>[2x]MTGPILSGLDPRFERTLYAHVGKEGSWTLDYYLRHGGYETAKRVLKEKTPDEVIEEVKRSGLRGRGGAGFPTGLKWSFMPKDDGKQHYLICNADESEPGSFKDRYILEDVPHLLIEGMILAGYAIRATVGYIYVRGEYRRAADRLEQAIKEARARGYLGKNLFGTDFSFDLHVHRGAGAYICGEETALMNSLEGLRANPRLKPPFPAQSGLWGKPTTINNVETLASVVPIMERGADWFAQMGTEQSKGMKLYQISGPVKRPGVYELPMGTTFRELIYEWAGGPLEPIQAIIPGGSSTPPLPFTEEVLDTPMSYEHLQAKGSMLGTGGVILIPERVSMVDAMWNLTRFYAHESCGKCTPCREGVAGFMVNLFAKIGTGQGEEKDVENLEALLPLIEGRSFCPLADAAVWPVKGSLRHFKDQYLALAREKRPVPRPSLWR;>MGFFDDKQDFLEETFAKYPPEGRRAAIMPLLRRVQQEEGWIRPERIEEIARLVGTTPTEVMGVASFYSYYQFVPTGKYHLQVCATLSCKLAGAEELWDYLTETLGIGPGEVTPDGLFSVQKVECLGSCHTAPVIQVNDEPYVECVTRARLEALLAGLRAGKRLEEIELPGKCGHHVHEVEV[2x];>[2x]MVRVKVNDRIVEVPPGTSVMDAVFHAGYDVPLFCSEKHLSPIGACRMCLVRIGLPKKGPDGKPLLNEKGEPEIQWQPKLAASCVTAVADGMVVDTLSDVVREAQAGMVEFTLLNHPLDCPTCDKGGACELQDRTVEYGLYEKYYQKGPLELPVYTRFEFTRRHVDKHHPLSPFVILDRERCIHCKRCVRYFEEVPGDEVLDFIERGVHTFIGTMDFGLPSGFSGNITDICPVGALLDLTARFRARNWEMEETPTTCALCPVGCGITADTRSGELLRIRAREVPEVNEIWICDAGRFGHEWADQNRLKTPLVRKEGRLVEATWEEAFLALKEGLKEARGEEVGLYLAHDATLEEGLLASELAKALKTPHLDFQGRTAAPASLFPPASLEDLLQADFALVLGDPTEEAPILHLRLSEFVRDLKPPHRYNHGTPFADLQIKERMPRRTDKMALFAPYRAPLMKWAAIHEVHRPGEEREILLALLGDKEGSEMVAKAKEAWEKAKNPVLILGAGVLQDTVAAERARLLAERKGAKVLAMTPAANARGLEAMGVLPGAKGASWDEPGALYAYYGFVPPEEALKGKRFVVMHLSHLHPLAERYAHVVLPAPTFYEKRGHLVNLEGRVLPLSPAPIENGEAEGALQVLALLAEALGVRPPFRLHLEAQKALKARKVPEAMGRLSFRLKELRPKERKGAFYLRPTMWKAHQAVGKAQEAARAELWAHPETARAEALPEGAQVAVETPFGRVEARVVHREDVPKGHLYLSALGPAAGLRVEGRVLVPAGGEA;>MREEFLEEIPLDAPPEEAKELRTEVMTLNVGPQHPSTHGVLRLMVTLSGEEVLEVVPHIGYLHTGFEKTMEHRTYLQNITYTPRMDYLHSFAHDLAYALAVEKLLGAVVPPRAETIRVILNELSRLASHLVFLGTGLLDLGALTPFFYAFRERETILDLFEWVTGQRFHHNYIRIGGVKEDLPEEFVPELKKLLEVLPHRIDEYEALFAESPIFYERARGVGVIPPEVAIDLGLTGGSLRASGVNYDVRKAYPYSGYETYTFDVPLGERGDVFDRMLVRIREMRESVKIIKQALERLEPGPVRDPNPQITPPPRHLLETSMEAVIYHFKHYTEGFHPPKGEVYVPTESARGELGYYIVSDGGSMPYRVKVRAPSFVNLQSLPYACKGEQVPDMVAIIASLDPVMGDVDR[2x];>MRLERVLEEARAKGYPIEDNGLGNLWVVLPRERFKEEMAHYKAMGFNFLADIVGLDYLTYPDPRPERFAVVYELVSLPGWKDGDGSRFFVRVYVPEEDPRLPTVTDLWGSANFLEREVYDLFGIVFEGHPDLRKILTPEDLEGHPLRKDYPLGETPTLFREGRYIIPAEFRAALTGKDPGLTFYKGGSRKGYRSLWADLKKAREVKG[2x];>MALKDLFERDVQELEREGILFTTLEKLVAWGRSNSLWPATFGLACCAIEMMASTDARNDLARFGSEVFRASPRQADVMIVAGRLSKKMAPVMRRVWEQMPDPKWVISMGACASSGGMFNNYAIVQNVDSVVPVDVYVPGCPPRPEALIYAVMQLQKKVRGQAYNERGERLPPVAAWKRTRG[2x];>MSASSERELYEAWVELLSWMREYAQAKGVRFEKEADFPDFIYRMERPYDLPTTIMTASLSDGLGEPFLLADVSPRHAKLKRIGLRLPRAHIHLHAHYEPGKGLVTGKIPLTKERFFALADRAREALAFA[2x];>[2x]MTLKALAQSLGITLKYLFSKPVTVPYPDAPVALKPRFHGRHVLTRHPNGLEKCIGCSLCAAACPAYAIYVEPAENDPENPVSAGERYAKVYEINMLRCIFCGLCEEACPTGAIVLGYDFEMADYEYSDLVYGKEDMLVDVVGTKPQRREAKRTGKPVKVGYVVPYVRPELEGFKAPTEGGKR;>MAPIQEYVGTLIYVGVALFIGVAALLVGALLGPKKPGRAKLMPYESGNDPAGEVKRFPVHFYVVAMLFILFDVEVAFLWPYAVSAGGLGLYGFLGVLAFTLLLFVGFLYEWWKGVMRWH[2x];>[2x]MTWSYPVDPYWMVALKALLVVVGLLTAFAFMTLIERRLLARFQVRMGPNRVGPFGLLQPLADAIKSIFKEDIVVAQADRFLFVLAPLISVVFALLAFGLIPFGPPGSFFGYQPWVINLDLGILYLFAVSELAVYGIFLSGWASGSKYSLLGSLRSSASLISYELGLGLALLAPVLLVGSLNLNDIVNWQKEHGWLFLYAFPAFLVYLIASMAEAARTPFDLPEAEQELVGGYHTEYSSIKWALFQMAEYIHFITASALIPTLFLGGWTMPVLEVPYLWMFLKIAFFLFFFIWIRATWFRLRYDQLLRFGWGFLFPLALLWFLVTALVVALDLPRTYLLYLSALSFLVLLGAVLYTPKPARKGGGA;>[2x]MSLLEGLALFLLLLSGVLVVTLRNAIHAALALILNFLVLAGVYVALDARFLGFIQVIVYAGAIVVLFLFVIMLLFAAQGEIGFDPLVRSRPLAALLALGVAGILAAGLWGLDLAFTQDLKGGLPQALGPLLYGDWLFVLLAVGFLLMAATVVAVALVEPGKASRAKEAEKREEVAR;>[2x]MSYLLTSALLFALGVYGVLTRRTAILVFLSIELMLNAANLSLVGFARAYGLDGQVAALMVIAVAAAEVAVGLGLIVAIFRHRESTAVDDLSELRG;>[2x]MALLGTILLPLLGFALLGLFGKRMREPLPGVLASGLVLASFLLGAGLLLSGGARFQAEWLPGIPFSLLLDNLSGFMLLIVTGVGFLIHVYAIGYMGGDPGYSRFFAYFNLFIAMMLTLVLADSYPVMFIGWEGVGLASFLLIGFWYKNPQYADSARKAFIVNRIGDLGFMLGMAILWALYGTLSISELKEAMEGPLKNPDLLALAGLLLFLGAVGKSAQIPLMVWLPDAMAGPTPVSALIHAATMVTAGVYLIARSSFLYSVLPDVSYAIAVVGLLTAAYGALSAFGQTDIKKIVAYSTISQLGYMFLAAGVGAYWVALFHVFTHAFFKALLFLASGSVIHALGGEQDVRKMGGLWKHLPQTRWHALIGALALGGLPLLSGFWSKDAILAATLTYPFGGVGFYVGALLVAVLTAMYAMRWFVLVFLGEERGHHHPHEAPPVMLWPNHLLALGSVLAGYLALPHPLPNVLEPFLKPALAEVEAHHLSLGAEWGLIALSAAVALLGLWAGFVFFQRKVFPAWYLAFEAASREAFYVDRAYNALIVNPLKALAEALFYGDRGLLSGYFGLGGAARSLGQGLARLQTGYLRVYALLFVLGALLLLGVMRW;>MVVLAVLLPVVFGALLLLGLPRALGVLGAGLSFLLNLYLFLTHPGGVAHAFQAPLLPGAGVYWAFGLDGLSALFFLTIALTVFLGALVARVEGRFLGLALLMEGLLLGLFAARDLLVFYVFFEAALIPALLMLYLYGGEGRTRALYTFVLFTLVGSLPMLAAVLGARLLSGSPTFLLEDLLAHPLQEEAAFWVFLGFALAFAIKTPLFPLHAWLPPFHQENHPSGLADALGTLYKVGVFAFFRFAIPLAPEGFAQAQGLLLFLAALSALYGAWVAFAAKDFKTLLAYAGLSHMGVAALGVFSGTPEGAMGGLYLLAASGVYTGGLFLLAGRLYERTGTLEIGRYRGLAQSAPGLAALALILFLAMVGLPGLSGFPGEFLTLLGAYKASPWLAALAFLSVIASAAYALTAFQKTFWEEGGSGVKDLAGAEWGFALLSVLALLLMGVFPGYFARGLHPLAEAFAKLLGGGA[2x];>MTLAILAVFSVALTLLGFVLPPQGVKRATLLGLALALASLLLTWGKPFAFGPYAVDGVSQVFTLLALLGALWTVGLVRSGRFEFYLLVLYAALGMHLLASTRHLLLMLVALEALSLPLYALATWRRGQGLEAALKYFLLGALAAAFFLYGAALFYGATGSLVLGAPGEGPLYALALGLLLVGLGFKAALAPFHFWTPDVYQGSPTPVVLFMATSVKAAAFAALLRVAAPPEALALLVALSVVVGNLAALAQKEAKRLLAYSSIAHAGYMALALYTGNAQALGFYLLTYVLATGLAFAVLSQISPDRVPLEALRGLYRKDPLLGLAFLVAMLSLLGLPPLAGFWGKYLAFAEAARAGAWGVLVLALVTSAVSAYYYLGLGLAVFARPEETPFRPGPPWARAAVVAAGVLLLALGLLPGLVLPALAAGG[2x];>MVRVGMRAAPRVSLEALKAALGGLKLSEAKVYLITDWQDKRDQARYALLLHTGKKDLLVPDAFGPAFPGGEEALSELVGLLLAQGARRFYEAVVSPGEMTALLDLPPEELLKRVMAIANPTDPGIYLKRAA[2x]

Complex I (NADH:ubiquinone (UQ) oxidoreductase) is the first and the largest enzyme of the respiratory chain, catalysing the transfer of two electrons from NADH to UQ, coupled to the translocation of four protons across the bacterial or inner mitochondrial membrane. In bacterial complex I the 14 “core” subunits, necessary and sufficient for complex I function, are shared equally between the peripheral and membrane arms, together forming an L-shaped molecule. All known co-factors of complex I reside in the PA: the primary electron acceptor flavin-mononucleotide (FMN) is connected by the redox chain of seven Fe–S clusters to the quinone-binding site (Q-site) at the interface with the membrane domain. In this work we address this question by building and analyzing atomic structures of nine different conformational states of complex I, which were obtained by X-ray crystallography and single-particle cryo-EM.

Aureothin, pyridaben and piericidin A are the most potent inhibitors of T. thermophilus complex I, while rotenone is less effective than it is with mammalian enzyme. All Q-like ligands studied here display a similar pattern of interactions at the deepest end of the Q-cavity, with the headgroup about 12 Å away from cluster N2. A shared feature between all ligands bound in the Q-site is a hydrogen bond interaction of a ketone group from the quinone ring with the conserved and essential for complex I activity Y87416,36. Finally, pyridaben seems to be stabilized only through the conserved interaction with Y874, although its proximity to Q334 (3–4 Å) could facilitate an interaction with both the thioether and chloride groups. In addition, the tert-butyl group points towards a small hydrophobic cavity and the 4-tert-butylcyclohexyl moiety is surrounded by non-polar residues, completing its accommodation. In these structures quinone-like compounds are bound in the main “deep” site within the cavity, where quinone can effectively accept electrons from cluster N2. Most dramatic changes are caused by DQ binding, whilst Q-like inhibitors alter complex I conformation consistently in a similar way but to a lesser degree, to states intermediate between CXIINT and CXIDQ. The overlap analysis (OA) (technique described below) shows that transitions from CXIINT structure to CXIAUT and CXIPYR involve relatively minor PA rotation component (mode 8), which is much stronger for CXIPIE structure and is accompanied in addition by a bending motion (mode 7) for CXIDQ structure.>[2x]GQANHPTAAVVTEKQQMLEQHLQDVRKRVQDLEQKMKVVENLQDDFDFNYKTLKSQGDMQDLNGNNQSVTRQKMQQLEQMLTALDQMRRSIVSELAGLLSAMEYVQKTLTDEELADWKRRQQIACIGGPPNICLDRLENWITSLAESQLQTRQQIKKLE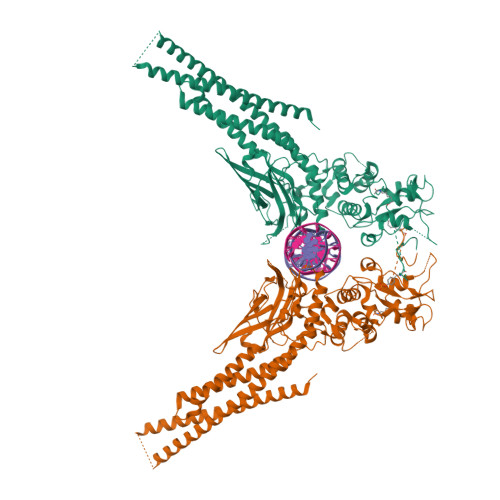ELQQKVSYKGDPIVQHRPMLEERIVELFRNLMKSAFVVERQPCMPMHPDRPLVIKTGVQFTTKVRLLVKFPELNYQLKIKVCIDKDSGDVAALRGSRKFNILGTNTKVMNMEESNNGSLSAEFKHLTLREQRCGNGGRANCDASLIVTEELHLITFETEVYHQGLKIDLETHSLPVVVISNICQMPNAWASILWYNMLTNNPKNVNFFTKPPIGTWDQVAEVLSWQFSSTTKRGLSIEQLTTLAEKLLGPGVNYSGCQITWAKFCKENMAGKGFSFWVWLDNIIDLVKKYILALWNEGYIMGFISKERERAILSTKPPGTFLLRFSESSKEGGVTFTWVEKDISGSTQIQSVEPYTKQQLNNMSFAEIIMGYKIMDATNILVSPLVYLYPDIPKEEAFGKYCRPESQEHPEADPGSAAPYLKTKFICVTPFIDAVWK(4-methyl-3-nitro-phenyl)-oxidanyl-oxidanylidene-boron 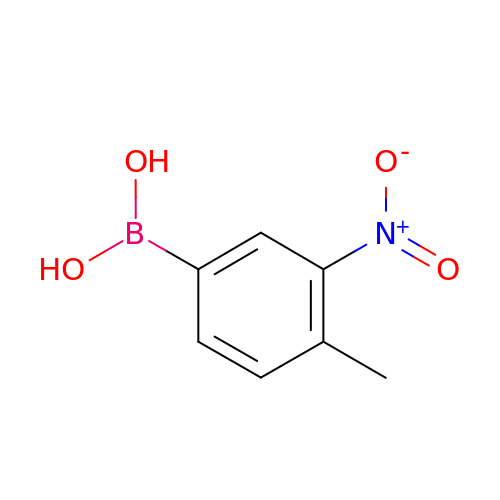| C7 H8 B N O4 | OASVXBRTNVFKFS-UHFFFAOYSA-N>MALRFEALYPEGMCPGWSVVVKGKTSSNTSMFEINFLSHPGDQIAFHFNPRFASSRIVCNSFLANHWGKEEVNKTFPFEAKEPFQVEIYSDQDYFHIFIDENKILQYKHRQKQLSSITKLQILNDIEISSVEITKRGLY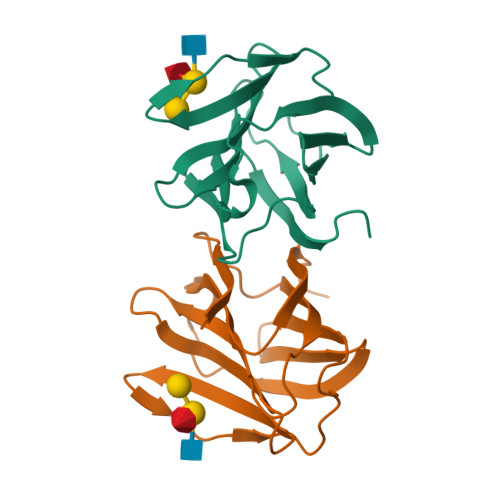[2x]> MGSSHHHHHHSSGLVPGSHMGGRPRQHLLSLTRRAQKHRLRELKIQVKEFAD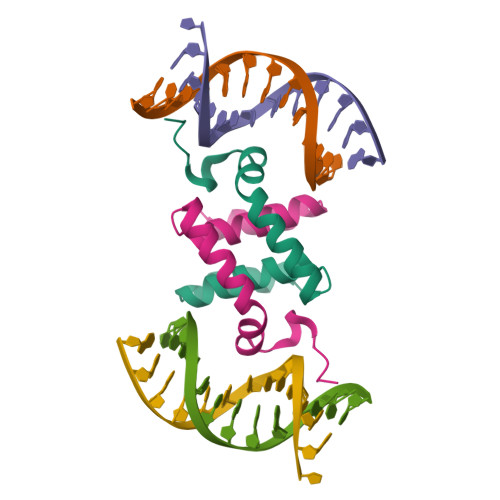KEEGGDVKAVCLTLFLLALRARNEHRQADELEAIMQGRGSGLQP> AAPTSSIEIVLDKTTASVGEIVTASINIKNITNFSGCQLNMKYDPAVLQPVTSSGVAYTKSTMP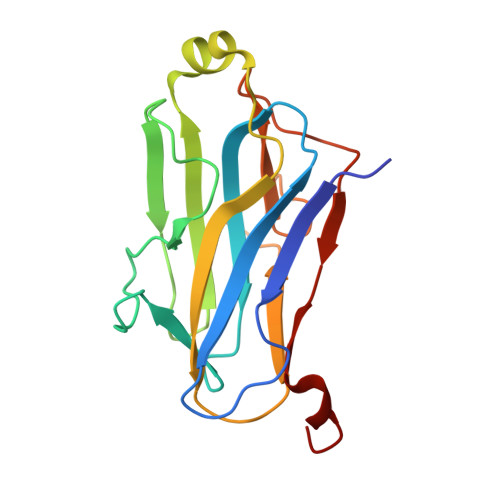GAGTILNSDFNLRQVADNDLEKGILNFSKAYVSLDDYRTAAAPEQTGTVAVVKFKVLKEETSSISFEDTTSVPNAIDGTVLFDWNGDRIQSGYSVIQPAVINLDMIKAS> SNAIAVGSERSADGKGMLLANPHFPWNGAMRFYQMHLTIPGRLDVMGASLPGLPVVNIGFSRHLAWTHTVDTSSHFTLYRLALDPKDPRRYLVDGRSLPLEEKSVAIEVRGADGKLSRVEHKVYQSIYGPLVVWPGKLDWNRSEAYALRDANLENTRVLQQWYSINQASDVADLRRRVEALQGIPWVNTLAADEQGNALYMNQSVVPYLKPELIPACAIPQLVAEGLPALQGQDSRCAWSRDPAAAQAGITPAAQLPVLLRRDFVQNSNDSAWLTNPASPLQGFSPLVSQEKPIGPRARYALSRLQGKQPLEAKTLEEMVTANHVFSADQVLPDLLRLCRDNQGEKSLARACAALAQWDRGANLDSG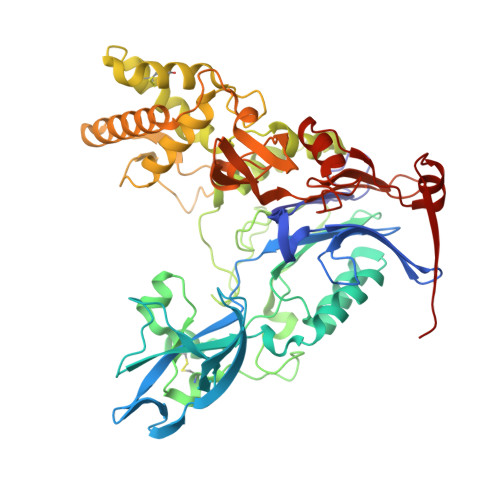SGFVYFQRFMQRFAELDGAWKEPFDAQRPLDTPQGIALDRPQVATQVRQALADAAAEVEKSGIPDGARWGDLQVSTRGQERIAIPGGDGHFGVYNAIQSVRKGDHLEVVGGTSYIQLVTFPEEGPKARGLLAFSQSSDPRSPHYRDQTELFSRQQWQTLPFSDRQIDADPQLQRLSIREAA>MNQNLLVTKRDGSTERINLDKIHRVLDWAAEGLHNVSISQVELRSHIQFYDGIKTSDIHETIIKAAADLISRDAPDYQYLAARLAIFHLRKKAYGQFEPPALYDHVVKMVEMGKYDNHLLEDYTEEEFKQMDTFIDHDRDMTFSYAAVKQLEGKYLVQNRVTGEIYESAQFLYILVAACLFSNYPRETRLQYVKRFYDAVSTFKISLPTPIMSGVRTPTRQFSSCVLIECGDSLDSINATSSAIVKYVSQRAGIGINAGRIRALGSPIRGGEAFHTGCIPFYKHFQTAVKSCSQGGVRGGAATLFYPMWHLEVESLLVLKNNRGVEGNRVRHMDYGVQINKLMYTRLLKGEDITLFSPSDVPGLYDAFFADQEEFERLYTKYEKDDSIRKQRVKAVELFSLMMQERASTGRIYIQNVDHCNTHSPFDPAIAPVRQSNLCLEIALPTKPLNDVNDENGEIALCTLSAFNLGAINNLDELEELAILAVRALDALLDYQDYPIPAAKRGAMGRRTLGIGVINFAYYLAKHGKRYSDGSANNLTHKTFEAIQYYLLKASNELAKEQGACPWFNETTYAKGILPIDTYKKDLDTIANEPLHYDWEALRESIKTHGLRNSTLSALMPSETSSQISNATNGIEPPRGYVSIKASKDGILRQVVP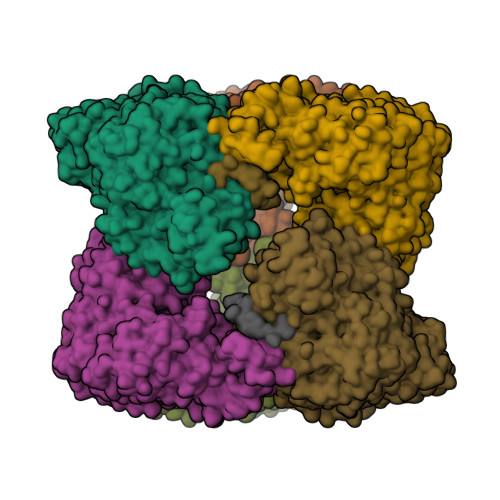DYEHLHDAYELLWEMPGNDGYLQLVGIMQKFIDQSISANTNYDPSRFPSGKVPMQQLLKDLLTAYKFGVKTLYFQNTRDGAEDAQDDLVPSIQDDGCESGACKI[3x];>[4x]YLVGQIDSEVDTDDLSNFQL> MALLLASAINHTAHPAGLRSHPNNESFSRHHLCSSPQNISKRRSNLSFRPRAQTISSESAGIHRLSPWEIPRRDWFPPSFLFGAATSAYQIEGAWNEDGKGPSTWDHFCHNFPEWIVDRSNGDVAADSYHMYAEDVRLLKEMGMDAYRFSISWPRILPKGTLAGGINEKRVEYYNKLIDLLLENGIEPYITIFHWDTPQALVDAYGGFLDERIIKDYTDFAKVCFEKFGKTVKNWLT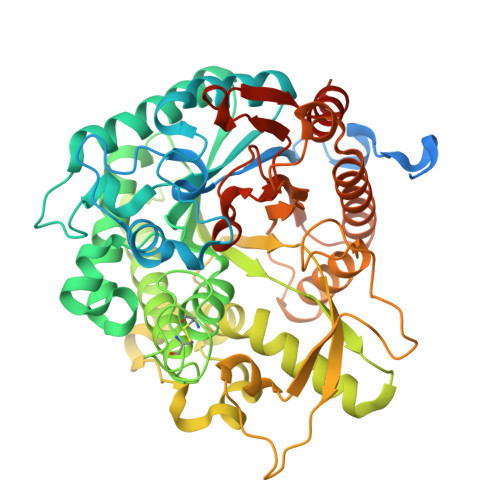FNEPETFCSVSYGTGVLAPGRCSPGVSCAVPTGNSLSEPYIVAHNLLRAHAETVDIYNKYHKGADGRIGLALNVFGRVPYTNTFLDQQAQERSMDKCLGWFLEPVVRGDYPFSMRVSARDRVPYFKEKEQEKLVGSYDMIGINYYTSTFSKHIDLSPNNSPVLNTDDAYASQETKGPDGNAIGPPTGNAWINMYPKGLHDILMTMKNKYGNPPMYITENGMGDIDKGDLPKPVALEDHTRLDYIQRHLSVLKQSIDLGADVRGYFAWSLLDNFEWSSGYTERFGIVYVDRENGCERTMKRSARWLQEFNGAAKKVENNKILTPAGQLN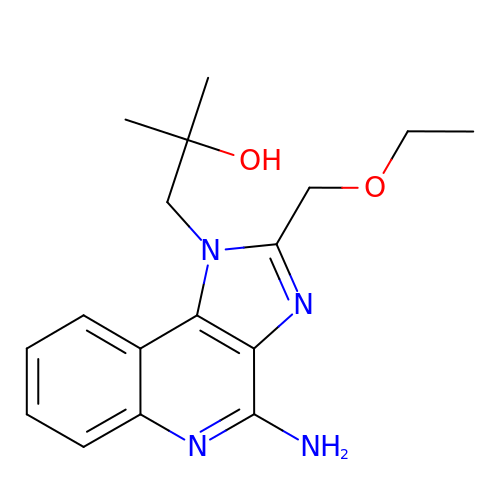1-[4-amino-2-(ethoxymethyl)-1H-imidazo[4,5-c]quinolin-1-yl]-2-methylpropan-2-ol | C17 H22 N4 O2 | BXNMTOQRYBFHNZ-UHFFFAOYSA-N>MGSSHHHHHHSQDPGINRKAINFDLSTKSLEKYFKDTREPYSLIKKFMLENGFEHRQYSGYTSKEPINERRVIRIINKLTKKFTWLGECVKEFDITEIGEQYSLKETIQDLCAKDFHQKLKEFTEKTPKNQKLKDLER[2x];>[2x]MASMTGGLEHPQFEKLEQKLISEEDLEDLAYPLLGTRIVLDEEKILKEGKYNLEDMYKMIDEYAKESGMIKINKETYHCKGDKYDLGCMTLFIYKYLIDSEWFTKNAKEWIWISEKEGNSDLISASKAEGEGIWE

Most TA systems are composed of two components—a toxin that impairs an essential process in the cell and a cognate antitoxin that restrains the toxin activity. The VapD proteins have a ferredoxin-like fold. The minimal nuclease-active form of VapDHpy and VapDHin is a dimer, with each subunit jointly forming a cleft that contains the putative catalytic site with conserved aspartate and serine residues. The VapW antitoxins are VapD homologs but lack the catalytic residues.

The structure was refined to an R factor of 0.221 and Rfree of 0.249 at 1.95 Å resolution. The asymmetric unit contains two VapD and two VapW molecules. As expected, both VapDCje and VapWCje adopt a modified ferredoxin-like fold (β1α1′α1β2β3α2α2′β4) characteristic of VapD and Cas2 proteins. However, while the α3 helix of VapDCje interacts with the core of another VapD subunit, the α3 of VapWCje interacts with its own core. As a result, VapW does not form homo- and heterodimers the way VapD and Cas2 do. While the two VapD molecules in the asymmetric unit do not form a homodimer, each of them forms homodimers related by a crystallographic twofold axis, resulting in two distinct VapD-VapW complexes with a 2:2 stoichiometry, designated as complexes 1 and 2. While the VapX antitoxin binds in the cleft between the two cognate VapD subunits and occludes the catalytic site, VapW binds on the opposite side of the VapD enzyme. In the VapD-VapW complex, the binding of the VapD toxin to the VapW antitoxin mimics the interactions between the dimers in the VapDHin hexamer. Each VapW chain simultaneously interacts with both VapD subunits. The crystal structure of the VapD-VapW complex indicates that VapW neither blocks the catalytic cleft of VapDCje nor disrupts homodimer formation.> MAISKTNGQSKPKRKTEVPGQALGYSLQFTLLTHLLLQAPEGSLCSLEVLDDVAQENNSGDIKFIQSKSALTANPAADRAKSLWKTLSNWIDLATSPDFEVEKAIFEL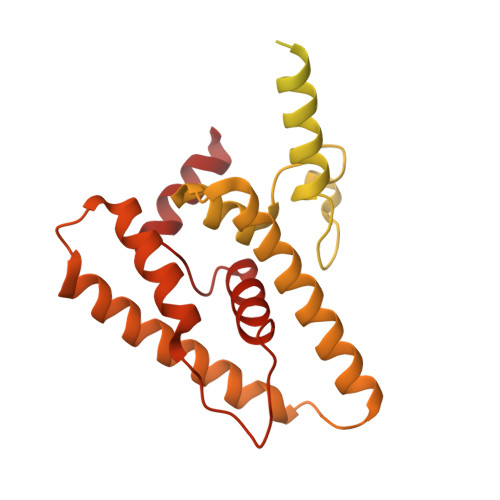YVSRPVEGSIVKKFNEAKTPEDAQEAITHARTELWGDSPHFTLKDGISKEISKYVEKVFTADQNLLQRLICNFQLTLGSGSPQADLEACVRSHPVSPSKVSDITNYLCGKVKRHIDMLLEAEKPAVIARDDFYTWYKAYVQKIDRQMVLSSRAQAPVKEKAQEYLPDKFVQQLEIIGLPYEEILGAISDYLMASFDRTDWAARGEVDETSFDDLDTALQRTWKNKQRICGLTHSEKSEQDQGKLLYFECMQFNIPLQAMSPPSHFIPGCYHILADSLAVGWHPNYTTQLKNKKVA The semaphorins are the largest family of evolutionarily conserved axon guidance cues. The semaphorins signal through their main receptors, plexins, which are single-spanning transmembrane proteins expressed in a variety of cell types, including neurons, cancer cells or endothelial cells. We determined crystal structures of Drosophila Sema1a1–2, Sema1b1–2, Sema2a1–3 and Sema2b1–3 to a 3.6-, 2.8-, 2.1- and 2.5 -Å resolution, respectively. All structures contain the sema domain composed of a seven-bladed β-propeller fold, which is followed by a PSI domain.

Sema1a has been reported initially as a repulsive guidance cue mediating the defasciculation of motor axon bundles in the fly embryo. The genetic analysis provided compelling evidence that PlexA is a neuronal receptor for both Sema1a and Sema1b12. In the crystal, Sema1a1–2, Sema2a1–3 and Sema2b1–3 form a disulfide-linked dimer, while Sema1b1–2 is a monomer and the lattice packing provides no evidence for Sema1b1–2 dimerization within the crystal. Our crystal structures of Drosophila semaphorins revealed that the dimeric architecture in Sema1a, Sema2a and Sema2b is covalently secured by an intermolecular sema-to-sema disulfide bond formed by a cysteine from each of the β4B–β4 C loops of the opposing chains (Cys279 in Sema2a). Conversely, mutation of the cysteine residue involved in dimerization in Sema1aecto to serine completely abrogated dimerization, and no dimer was detected up to a concentration of 2 mg/ml. Despite the low propensity to non-covalently dimerize, Sema1aecto maintains the homodimeric architecture by reason of the covalent interchain disulfide bond. In class 1 semaphorins, two distinct loops with no obvious structural and functional role are substantially extended from the bottom face of the β-propeller, β5A–β5B and β7A–β7B in Sema1a, and β2C–β2D and β6C–β6D Sema1b. In the Sema1b ectodomain, the β2C–β2D loop is significantly extended while the β7A–β7B loop is extended in Sema1a. The linker in Sema1a is shorter by 35 residues compared with that of Sema1b.

>[2x]ETGYGPEDVLKFVGNESVVDHFKLVTKDGNSLLIGARNTVFNLSIHDLVEQQRLVWTSPEDDTKMCLVKGKDEEACQNYIRIMVVPSPGRLFVCGTNSFRPMCNTYIISDSNYTLEATKNGQAVCPYDPRHNSTSVLADNELYSGTVADFSGSDPIIYREPLQTEQYDSLSLNAPNFVSSFTQGDFVYFFFRETAVEFINCGKAIYSRVARVCKWDKGGPHRFRNRWTSFLKSRLNCSIPGDYPFYFNEIQSASNLVEGQYGSMSSKLIYGVFNTPSNSIPGSAVCAFALQDIADTFEGQFKEQTGINSNWLPVNNAKVPDPRPGSCHNDSRALPDPTLNFIKTHSLMDENVPAFFSQPILVRTSTIYRFTQIAVDAQIKTPGGKTYDVIFVGTDHGKIIKSVNAESADSADKVTSVVIEEIDVLTKSEPIRNLEIVRTMQYDQPKDGSYDDGKLIIVTDSQVVAIQLHRCHNDKITSCSECVALQDPYCAWDKIAGKCRSHGAPRWLEENYFYQNVATGQHAACPSGTKHHHHHH> 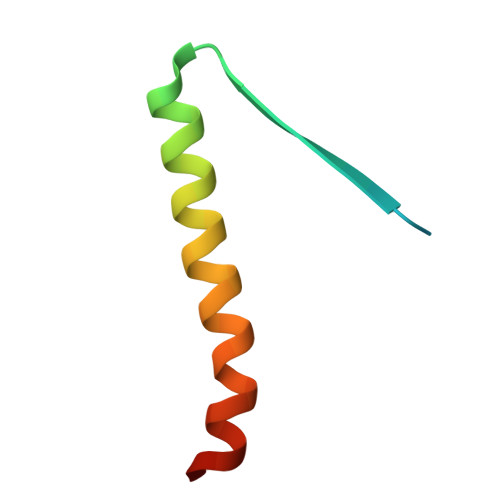MADIIADADSPAKITIKANKLKDLKDYVDDLKTYNNTYSNVVLEHHHHHH>[4x]MEGISIYTSDNY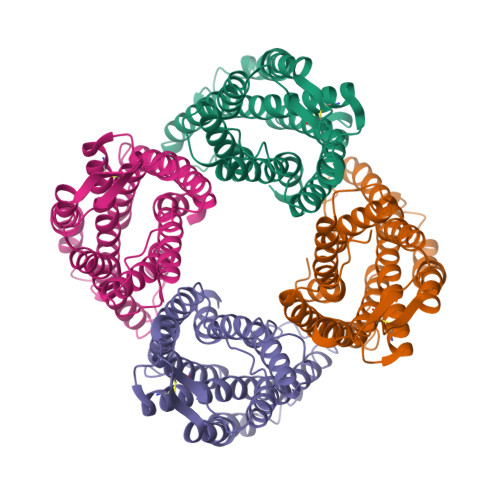TEEMGSGDYDSMKEPCFREENANFNKIFLPTIYSIIFLTGIVGNGLVILVMGYQKKLRSMTDKYRLHLSVADLLFVITLPFWAVDAVANWYFGNFLCKAVHVIYTVNLYSSVLILAFISLDRYLAIVHATNSQRPRKLLAEKVVYVGVWIPALLLTIPDFIFANVSEADDRYICDRFYPNDLWVVVFQFQHIMVGLILPGIVILSCYCIIISKLSHSKGHQKRKALKTTVILILAFFACWLPYYIGISIDSFILLEIIKQGCEFENTVHKWISITEALAFFHCCLNPILYAFLGAKFKTSAQHALTSVSRGSSLKILSKGKRGGHSSVSTESESSSFHSSDYKDDDDK>MDDAVARAVEIVRKQGVADANLVRMGDKSIMFSEKGDAFIMYGKQGRSWIALFDPVGPRQALPDLIWRFVETARAAGCRSVFYQISPALLSYCADAGLRAFKLGELAVVNLANFELKGGKWANLRQTASRAVRDGLEFAVIEPQDIPDVLDQLAHVSDTWLADHNAKEKSFSLGAFDPDYVCSQPVGVLKKDGKIVAFANILMTETKEEGSVDLMR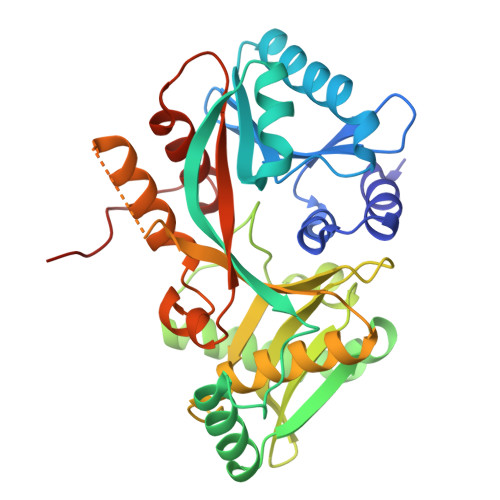FSPDAPKGSMDFLFVQILEYLKGEGFQRFNLGMAPLSGMSRRESAPVWDRVGGTVFEHGERFYNFKGLRAFKSKFHPEWQPRYLAVSGGVSPMIALMDATFLIGGGKLAAALEHHHHHH[2x]>IVGGYNCEENSVPYQVSLNSGYHFCGGSLINEQWVVSAGHCYKSRIQVRLGEHNIEVLEGNEQFINAAKIIRHPQYDRKTLNNDIMLIKLSSRAVINARVSTISLPTAPPATGTKCLISGWGNTASSGADYPDELQCLDAPVLSQAKCEASYPGKITSNMFCVGFLEGGKDSCQGDAGGPVVCNGQLQGVVSWGDGCAQKNKPGVYTKVYNYVKWIKNTIAANS[2x];>[2x]DSLGREAKCYNELNGCTKIYDPVCGTDGNTYPNECVLCFENRKRQTSILIQKSGPC

(1) The serine protease inhibitor Kazal type 1 (SPINK1) inhibits trypsin activity in zymogen granules of pancreatic acinar cells. TRY1 adopts the typical serine protease fold containing two β-barrels sandwiching the active site cleft of the protease. The inhibitor assumes a typical Kazal domain structure with a reactive loop surrounding a central α-helix. SPINK1 binds on top of the TRY1 p.S200A active site in a substrate-like manner, creating an interface of almost 1000 Å2.

We solved the crystal structures of TRY1 p.S200A bound to SPINK1 WT and p.N34S at 2.9 and 2.1 Å resolution, respectively. Similar to other known Laskowski-inhibitors, both SPINK1 variants bind to TRY1 p.S200A in a substrate-like manner. The specificity determining P1 residue Lys41 is oriented in a way that interacts with Asp194 in TRY1. The oxygen of the carbonyl carbon is stabilized by the oxyanion hole formed by the backbone nitrogen atoms of Ala200 and Gly198. In the present structure, Ser200 is replaced by an alanine to avoid proteolytic cleavage of the inhibitor or the protease due to residual protease activity observed even in the inhibitor bound complex. Unexpectedly, His63 exhibits an uncommon rotamer conformation, pointing outward and away from the catalytic triad. Instead, it points toward the sulfate ion bound within the SPINK1 loop. With this uncommon histidine conformation, TRY1 would not be able to catalyze the cleavage of the P1-P1′ scissile bond, as His63 could not function as a proton acceptor for Ser200, thereby not creating the strongly nucleophilic alkoxide ion. To analyze the impact of SPINK1 binding on the catalytic triad, we employed molecular dynamics simulations by using TRY1 WT and SPINK1 WT complexes, with His63 starting in either gauche+ or trans (Chi1 = 60° or 180°) conformation. SPINK1 binding sterically blocks the His63 rotamer conformation to flip from one state to the other most of the time.> MHHHHHHMKNVIFEDEEKSKMLARLLKSSHPEDLRAANKLIKEMVQEDQKRMEKISKRVN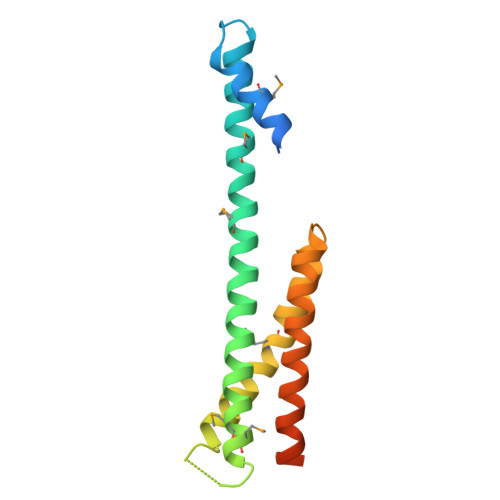AIEEVNNNVKLLTEMVMSHSQGGAAAGSSEDLMKELYQRCERMRPTLFRLASDTEDNDEALAEILQANDNLTQVINLYKQLVRGEEVNGDATAGSIPG> GHHHHHH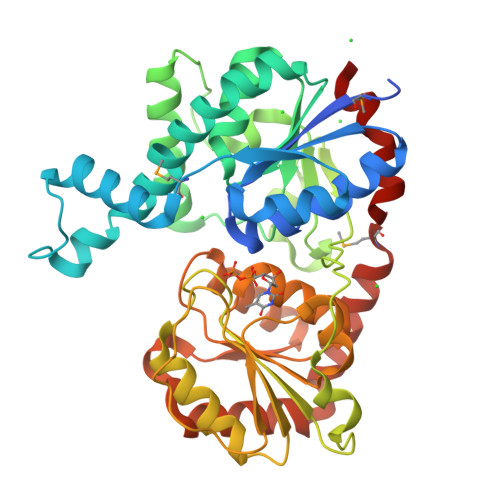HHHHSSGHIEGRHMRVLFASLGTHGHTYPLLPLATAARAAGHEVTFATGEGFAGTLRKLGFEPVATGMPVFDGFLAALRIRFDTDSPEGLTPEQLSELPQIVFGRVIPQRVFDELQPVIERLRPDLVVQEISNYGAGLAALKAGIPTICHGVGRDTPDDLTRSIEEEVRGLAQRLGLDLPPGRIDGFGNPFIDIFPPSLQEPEFRARPRRHELRPVPFAEQGDLPAWLSSRDTARPLVYLTLGTSSGGTVEVLRAAIDGLAGLDADVLVASGPSLDVSGLGEVPANVRLESWVPQAALLPHVDLVVHHGGSGTTLGALGAGVPQLSFPWAGDSFANAQAVAQAGAGDHLLPDNISPDSVSGAAKRLLAEESYRAGARAVAAEIAAMPGPDEVVRLLPGFASRSAG4-[[(2-methoxy-5-methyl-phenyl)sulfonylamino]methyl]-4-phenyl-N-(p-tolylmethyl)piperidine-1-carboxamide | C29 H35 N3 O4 S | 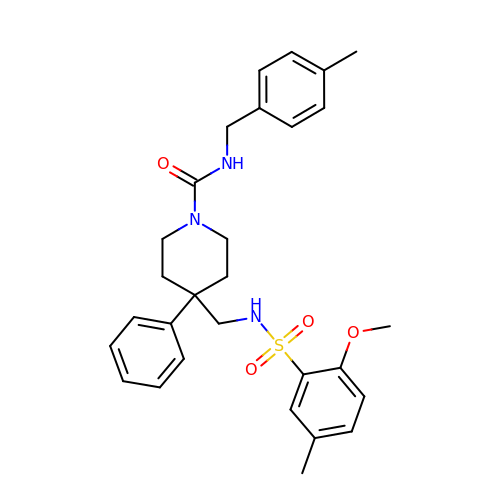ASTQWJGBKMEGSZ-UHFFFAOYSA-N RBcel1, an endoglucanase of the GH5_5 subfamily isolated from an uncultured bacterium, has aroused interest because of its ability to polymerize cellooligosaccharides in vitro under near-physiological conditions. After the glycosylation step, the donor sugar is covalently bound to the enzyme within its negatively numbered subsites. Transglycosylation occurs when a sugar hydroxyl group is used as an acceptor instead of a water molecule during the deglycosylation step. Solving the structures of two RBcel1 variants, RBcel1_E135Q and RBcel1_Y201F, in complex with ligands has brought to light some of the molecular factors behind transglycosylation.

Our previous study of RBcel1 showed that the substitution of Tyr201 with a phenylalanine residue drastically slows the deglycosylation step, resulting in accumulation of the GEI. A Tris molecule resides in the −1 subsite, as in the structure of RBcel1_WT. The structure of RBcel1_Y201F co-crystallized with G3 contains four monomers per asymmetric unit, with each monomer containing ligands ranging from G2 to G6 in the catalytic cleft. The presence of cellooligosaccharides longer than G3 within the negatively numbered subsites provides crystallographic evidence for transglycosylation. Several water molecules were placed in the model, but they are not sufficient to account for this excess of density. However, the presence of G6 in the negatively numbered subsites of RBcel1 in monomer B allowed the definition of two additional subsites: −5 and −6. As discussed in our previous study, a displacement of the Glu245 side chain to form the GEI, adopting the tt0° conformation instead of mt-10°, results in a change of electronic environment. In the structure of RBcel1_Y201F in complex with G3, the same displacement of the side chain of Glu245 was observed in monomers A, B and D, where a ligand is covalently bound. In monomer C, however, a G3 molecule occupies the +1 to +3 subsites, as in the structure of RBcel1_E135Q.

>SVDLIGINVAGAEFTGGKLPGKHGTHYFFPPEGYFEYWSEQGIHTVRFPLKWERLQPSLNAELDDVYASLVDDMLDQAKENDIKVILDVHNYARYRKKVIGTEDVPVSAYQDLMERIAKRWQGHDALFAYDIMNEPYGSADKLWPAAAQAGIDGVRKYDKKRPLLIEGASWSSAARWPRYADELLKLKDPADNMVFSAHVFIDEDASGSYKKGPGKDFEPMIGVKRVEPFVNWLKEHGKKGHIGEFGIPNDDERWLDAMDKLLAYLNENCIPINYWAAGPSWGNYKLSIEPKDGEKRPQVALLKKYAAKDNCSDFGPAKAE[4x]> GAMGLPGAEEAPVRVALRVRPLLPKELLHGHQSCLQVEPGLGRVTLGRDRHFGFHVVLAEDAGQEAVYQACVQPLLEAFFEGFNATVFAYGQTGSGKTYTMGEASVASLLEDEQGIVPRAMAEAFKLIDENDLLDCLVHVSYLEVYKEEFRDLLEVGTASRDIQLREDERGNVVLCGVKEVDVEGLDEVLSLLEMGNAARHTGATHLNHLSSRSHTVFTVTLEQRGRAPSRLPRPAPGQLLVSKFHFVDLAGSERVLKTGSTGERLKESIQINSSLLALGNVISALGDPQRRGSHIPYRDSKITRILKDSLGGNAKTVMIACVSPSSSDFDETLNTLNYASRAQ

Kif7, a member of the kinesin 4 superfamily, is implicated in a variety of diseases including Joubert, hydrolethalus and acrocallosal syndromes. It is also involved in primary cilium formation and the Hedgehog signalling pathway and may play a role in cancer. Members of the kinesin superfamily of motor proteins (Kifs) move unidirectionally along microtubules (MTs) in an ATP-dependent manner. Kif7, a critical regulator of mammalian Hh signalling, acts as both a positive and negative regulator in the Hh signalling pathway but performs this role differently from Cos2 in that it does not interact with Smo or Fu.

In our effort to characterize human kinesins of medical interest, we report here the crystal structure of the human Kif7 motor domain to 1.6 Å resolution. Of the seven Kif7 and Kif27 constructs used for crystallization, only Kif78–347, which lacks the neck linker region, yielded crystals. Kif78–347 crystallized as a monomer with one molecule per asymmetric unit. Data were collected to 1.6 Å resolution and the structure thus belongs to a small group of kinesins solved to a higher resolution. The final structure included residues 12–347 (missing regions: 107–114, 207–211, 230–241, 260–273) with bound Mg2+ADP (octahedrally co­ordinated) in the catalytic site and 328 water molecules. Kif7 contains an eight-stranded β-sheet core with three major solvent-exposed α-helices on each side, displaying the characteristic arrowhead-like structure typical of all members of the kinesin superfamily solved to date. Alignment of Kif78–347 with conventional kinesin (Kif5b) revealed their high structural similarity. In Kif5b the switch I region (residues 199–205) consists of a small helix (α3a), whereas in Kif7 it forms a loop (L9). The switch II cluster (helix α4/loop L12/helix α5) is in the so-called ‘down’ or ‘obstructive’ position and one would expect the neck linker (Arg350–Asn356) to be either unstructured or structured but in an undocked position with respect to the motor domain. Kif78–361 contained the neck-linker region but did not crystallize, whereas Kif78–347 lacking the neck linker revealed that the C-terminal residue Gln347 shows crystal contacts indicating that there would not be space for a neck linker in this crystal form.> MELPCAYGLLLHPT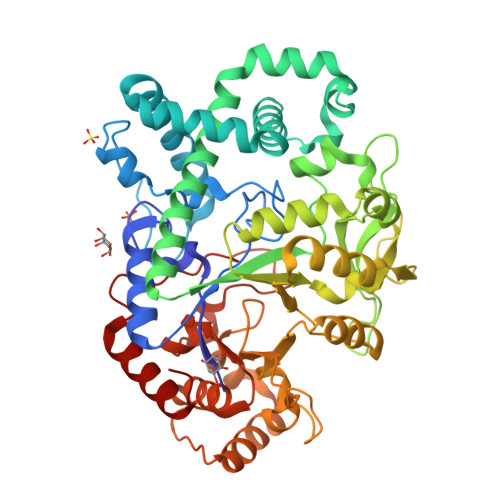SLPGPWGVGVLGEEARGFLRFLKEAGARYWQVLPLGPTGYGDSPYQSFSAFAGNPYLIDLRPLVDRGFVRLEDPGFPEGRVDYGLLYAWKWPALRAAFQGFRQKASPEEKEDFARFQEEEAWWLRDYALFMTLKSHHGGLPWNAWPLALRTREERALKEAEASLAEEIAFHAFTQWLFFRQWGALKEEAEALGIAFIGDMPIFVAEDSAEVWAHPEWFHLDEEGRPTVVAGVPPDYFSETGQRWGNPLYRWEVLEEEGFSFWIARLRKALELFHLVRIDHFRGFEAYWEIPASCPTAVEGRWVKAPGEKLFARIQEAFGRIPILAEDLGVITPEVEALRDRFGLPGMKVLQFAFDNGMENPFLPHNYPEHGRVVVYTGTHDNDTTLGWYRTATPHERDFLKRYLADWGITFREEAEVPWALMRLGMASRARLAVYPVQDVLALGSEARMNYPGRPSGNWAWRLRPGEIKEEHGERLLSLAEATGRV>MNLIPTVIETTNRGERAYDIYSRLLK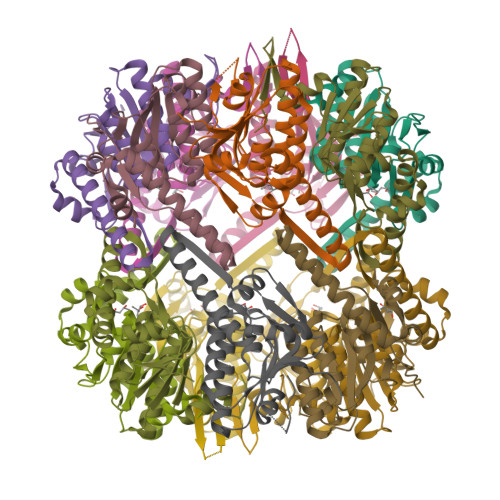DRIIMLGSQIDDNVANSIVSQLLFLQAQDSEKDIYLAINSPGGSVTAGFAIYDTIQHIKPDVQTICIGMAASMGSFLLAAGAKGKRFALPNAEVMIHQPLGGAQGQATEIEIAANHILKTREKLNRILSERTGQSIEKIQKDTDRDNFLTAEEAKEYGLIDEVMVPETK[14x]>GPDAETTTHPEAFQESLKHLLPDLSAYSEITIHLLHQLVLACGDVSLVNAVRLSQGAIASARDALKAGCPVVTDVPVVAAALDQTRLAHLGCTVKTLIDDPHITGLREAEQAFWHHDHWQQRLQQIPQGSVLAIGYAPSVLLTACKLIEQQHIQPALVIGMPIGF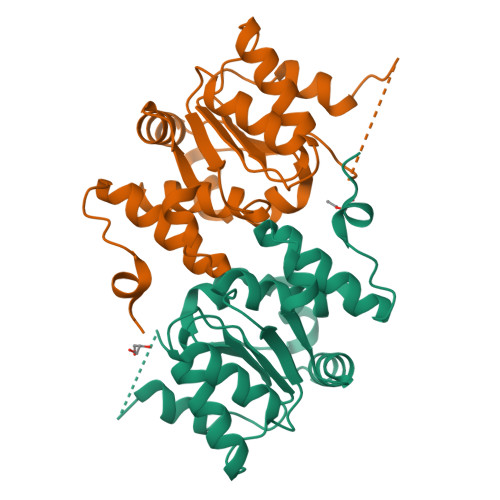SHAPGAKRRLMTSPIPHITIQGSLGGGLLAAVTLNALVETLIAKPDSHSYLTS[2x]> AATQQEIGKNMWDPFQSMRAVTGLMELTSGQCTQLS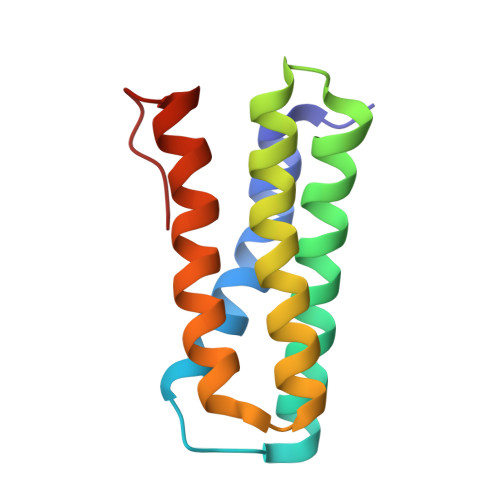KDAAAILAGVKESHDSISVDKNYKVLNDEVAYHAANIDAAAKANDLEEVQVQFRRMTIACRNCHKIYKTEQRLVP> TLSILVAHDLQRVIGFENQLPWHLPNDLKNVKKLSTGHTLVMGRK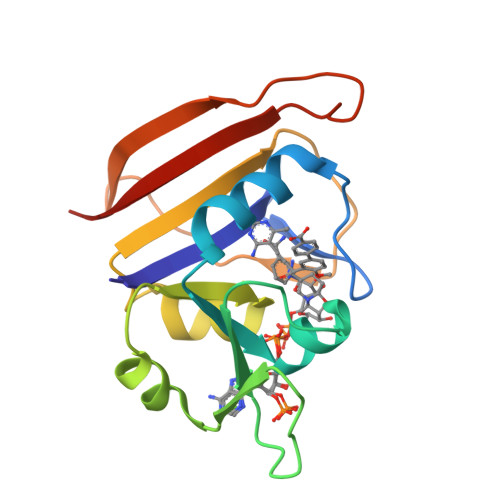TFESIGKPLPNRRNVVLTSDTSFNVEGVDVIHSIEDIYQLPGHVFIFGGQTLFEEMIDKVDDMYITVIEGKFRGDTFFPPYTFEDWEVASSVEGKLDEKNTIPHTFLHLIRKLEH>MGSSHHHHHHSSGLVPRGSHTGAGLRWKHTSSLKVANEPVLAFTQGSPERDALQKALKDLKGRMEAIPCVVGDEEVWTSDVQYQVSPFNHGHKVAKFCYADKSLLNKAIEAALAARKEWDLKPIADRAQIFLKAADMLSGPRRAEILAKTMVGQGKTVIQAEIDAAAELIDFFRFNAKYAVELEGQQPISVPPSTNSTVYRGLEGFVAAISPFNFTAIGGNLAGAPALMGNVVLWKPSDTAMLASYAVYRILREAGLPPNIIQFVPADGPLFGDTVTSSEHLCGINFTGSVPTFKHLWKQVAQNLDRFHTFPRLAGECGGKNFHFVHRSADVESVVSGTLRSAFEYGGQKCSACSRLYVPHSLWPQIKGRLLEEHSRIKVGDPAEDFGTFFSAVIDAKSFARIKKWLEHARSSPSLTILAGGKCDDSVGYFVEPCIVESKDPQEPIMKEEIFGPVLSVYVYPDDKYKETLQLVDSTTSYGLTGAVFSQDKDVVQEATKVLRNAAGNFYINDKSTGSIVGQQPFGGARASGTNDKPGGPHYILRWTSPQVIKETHK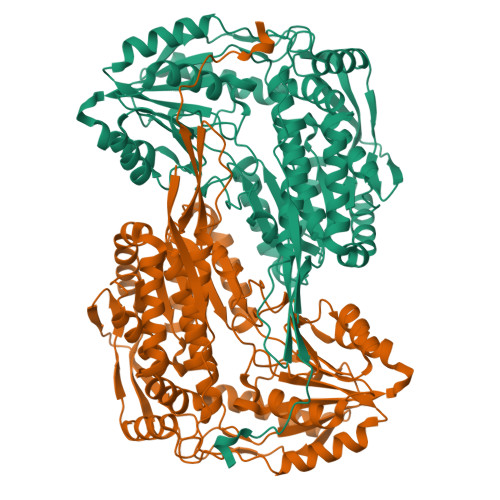PLGDWSYAYMQ[4x]> MKSTEKKELSHFRLKLETYLNEHFPEMSGNNPFITARSDEALTAYCDAVAQGFSHPEAESMASEVLYQGLHFSRYDTLVSVLEREFEQELPSPLPERLAPILLKNKAIQSVFAKYDLTDDFEASPEYEHLYTELTGTIVLLIESNHLPTIGG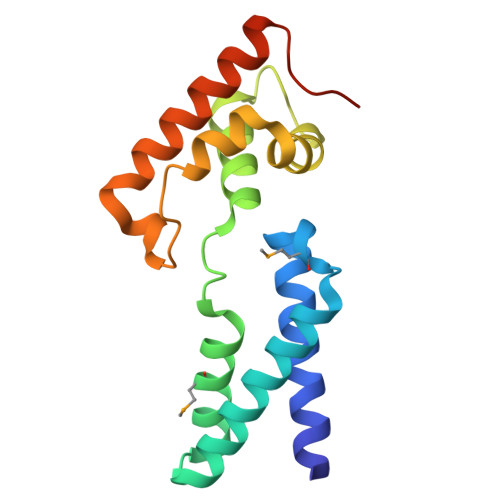GNDTV> SMDKKSLYKYLLLRSTGDMRRAKSPTIMTRVTNNVYLGNYKNAMNAPSSEVKFKYVLNLTMDKYTLPNSNINIIHIPLVDDTTTDISKYFDDVTAFLSKCDQRNEPVLVHCVAGVNRSGAMILAYLMSKNKESSPMLYFLYVYHSMRDLRGAFVENPSFKRQIIEKYVID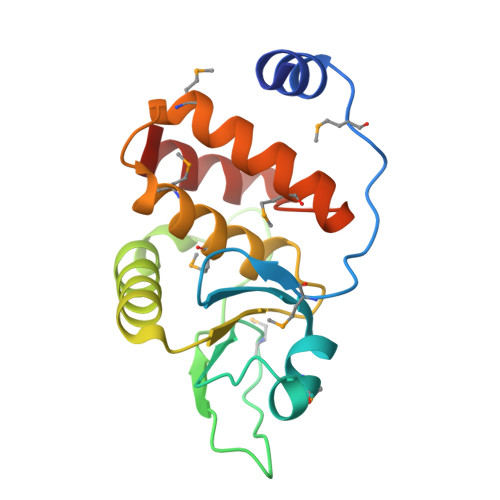KN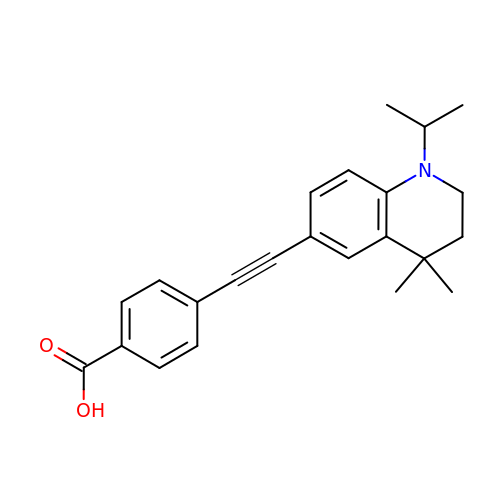4-[2-(4,4-dimethyl-1-propan-2-yl-2,3-dihydroquinolin-6-yl)ethynyl]benzoic acid | C23 H25 N O2 | OCMSZODRCJAGHL-UHFFFAOYSA-N>[2x]GPTITETSKPTLRRIPRSAGDEAIFQVLQEDGVVVIEGFMSADQVRRFNGEIDPHMKQWELGQKSYQESYLAGMRQLSSLPLFSKLFRDELMNDELLHGLCKRLFGPESGDYWLTTSSVLETEPGYHGQELHREHDGIPICTTLGRQSPESMLNFLTALTDFTAENGATRVLPGSHLWEDFSAPPPKADTAIPAVMNPGDAVLFTGKTLHGAGKNNTTDFLRRGFPLIMQSCQFTPVEASVALPRELVETMTPLAQKMVGWRTVSAKGVDIWTYDLKDLATGIDLKSNQVAKKA

EasH from Aspergillus japonicus (Aj_EasH) is a recently discovered enzyme involved in the biosynthesis of the natural product cycloclavine 4.1,2 This compound is a member of the ergot alkaloids, a fungal-derived class of natural products with a wide range of biological activities and pharmaceutical applications. Aj_EasH is a non-heme iron, α-keto-glutarate (aKG) dependent oxidase that works together with a flavoenzyme (EasA) and an NADPH-dependent oxidoreductase (EasG). In concert, these three enzymes catalyze the conversion of chanoclavine-I aldehyde 1 to cycloclavine 4. Aj_EasH catalyzes a highly unusual ring rearrangement to form the 5-3 ring system of the ergot alkaloid cycloclavine 4.

Subsequently, EasH was crystallized in 0.01 M ZnCl2 0.1 M HEPES pH 7.0, 20% (w/v) PEG 6000 and 1 mM aKG. Numerous efforts to soak or co-crystallize Aj_EasH with substrate (chanoclavine-I aldehyde 1) or product (cycloclavine 4) did not result in the observation of a ternary complex. However, the location of the active site could be clearly inferred from the location of the iron and aKG cofactors. The aKG appeared to be coordinated to the iron as would be expected for a catalytically competent orientation. The iron in Aj_EasH is coordinated by H131, E133, H209, in a similar fashion to AsqJ (H134, D136, H211) and Cp_EasH (H141, D143, H217). Within this loop there is a short helical segment (residues 52–72), which we refer to as the “lid”. The lid fully occludes the active site of Aj_EasH. Our X-ray structure reveals that the likely substrate binding pocket of Aj_EasH is spacious and largely hydrophobic (the pocket is delimited by Tyr65, Tyr69, Val236, Thr115, Leu119, Leu275, Leu70, Ile227 and Gly136) and, based on the relatively high B factors for the lid (residues 52–72), most probably highly plastic (Fig. SI-2.6, ESI†). However, given the hydrophobic active site environment and the lack of an acidic residue that could act to protonate any leaving group (Cl or OH) at carbon 10, an alternative mechanism of direct abstraction of hydrogen at C10 by the iron–oxo species followed by rearrangement should also be considered. A neutral, radical reaction intermediate is most consistent with the structure of the active site provided by this crystallographic study.> QEFEKVELTADGGVIKTILKKGDEGEENIPKKG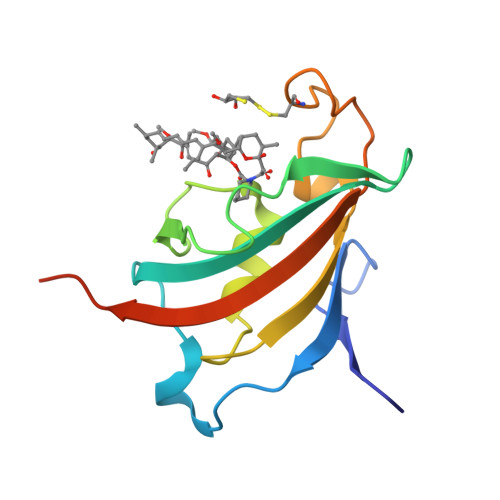NEVTVHYVGKLESTGKVFDSSFDRNVPFKFHLEQGEVIKGWDICVSSMRKNEKCLVRIESMYGYGDEGCGESIPGNSVLLFEIELLSFRELEETSHHHHHH> GGASRSVIRSIIKSSR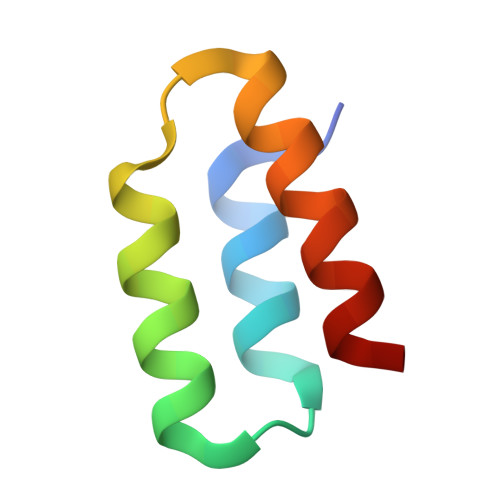LEEDRKRYLMTLLDDIKGANDLAKFHQMLMKIIMK> MENSEKTEVVLLACGSFNPITNMHLRLFELAKDYMNGTGRYTVVKGIISPVGDAYKKKGLIPAYHRVIMAELATKNSKWVEVDTWESLQKEWKETLKVLRHHQEKLEASDCDHQQNSPTLERPGRKRKWTETQDSSQKKSLEPKTKAVPKVKLLCGADLLESFAVPNLWKSEDITQIVANYGLICVTRAGNDAQKFIYESDVLWKHRSNIHVVNEWFANDISSTKIRRALRRGQSIRYLVPDLVQEYIEKHNLYSSESEDRNAGVILA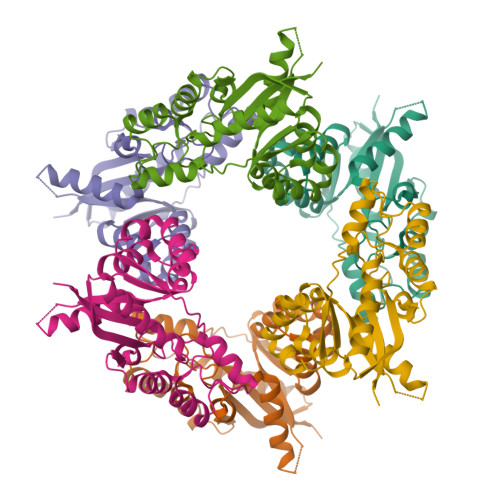PLQRNTAEAKT> SPSAEECGYSDRVRSITLGNSTITTQECANVVVAYGRWPEYLSDKEATAEDQPTQPDVATCRFYTLESVTWEKDSPGWWWKFPDALKDMGLFGQNMYYHYLGRAGYTIHVQCNASKFHQGCLLVVCVPEAEMGCSDVGGTVNEHAISEGEIAKKFSATATNGAHTVQSIVTNAGMGVGVGNLTIYPHQWVNLRTNNSATIVMPYINSVPMDNMFRHHNFTLMIIPFVSLDY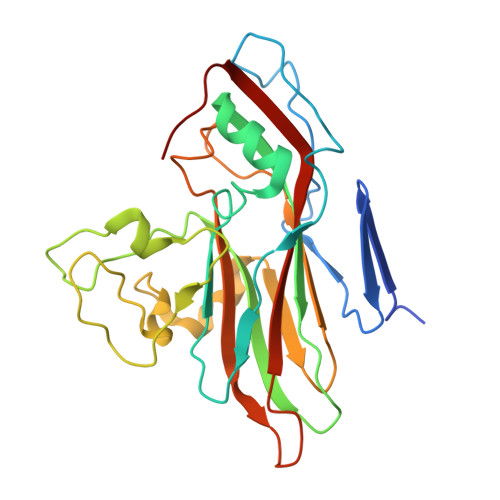SSDASTYVPITVTVAPMCAEYNGLRLATSLQ hexadecanethial 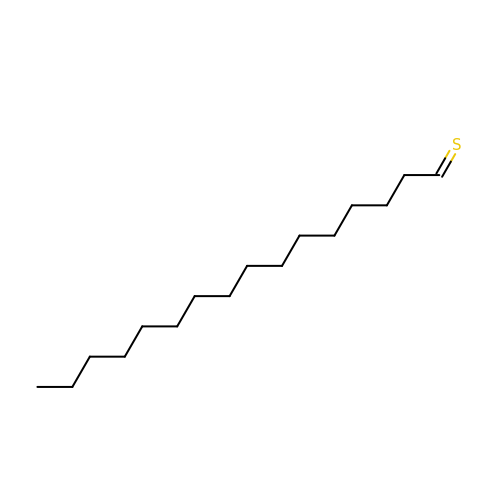| C16 H32 S | RPVPMVLNCKLUBI-UHFFFAOYSA-N>[8x]VDSVYRTRSLGVAAEGLPDQYADGEAARVWQLYIGDTRSRTAEYKAWLLGLLRQHGCHRVLDVACGTGVDSIMLVEEGFSVMSVDASDKMLKYALKERWNRRKEPSFDNWVIEEANWLTLDKDVLSGDGFDAVICLGNSFAHLPDCKGDQSEHRLALKNIASMVRPGGLL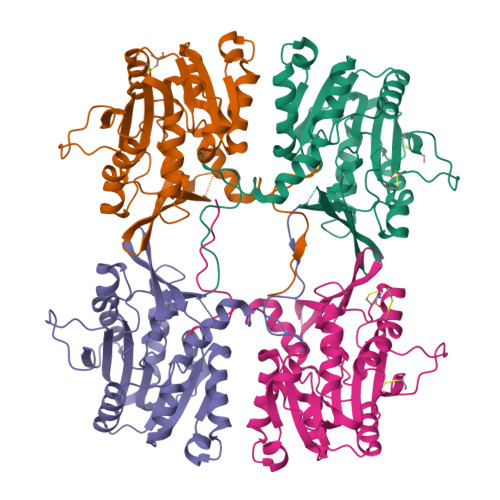VIDHRNYDYILSTGCAPPGKNIYYKSDLTKDITTSVLTVNNKAHMVTLDYTVQVPGTGRDGSPGFSKFRLSYYPHCLASFTELVRAAFGGRCQHSVLGDFKPYKPGQAYVPCYFIHVLKKTD> GSHMGSPNSPLKDSLRPKLSEEQQHIIAILLDAHHKTYDPTYADFRDFRPPVRMDGSTGSVTLDLSPLSMLPHLADLVSYSIQKVIGFAKMIPGFRDLTSDDQIVLLKSSAIEVIMLLSNQSFTMDDMSWDCGSQDYKYDVTDVSKAGHTLELIEPLIKFQVGLKKLNLHEEEHVLLMAICIVSPDRPGVQDAKLVEAIQDRLSNTLQTYIRCRHPPPGSHQLYAKMIQKLADLRSLNEEHSKQYRSLSFQPENSMKLTPLVLEVFGNEIS;> K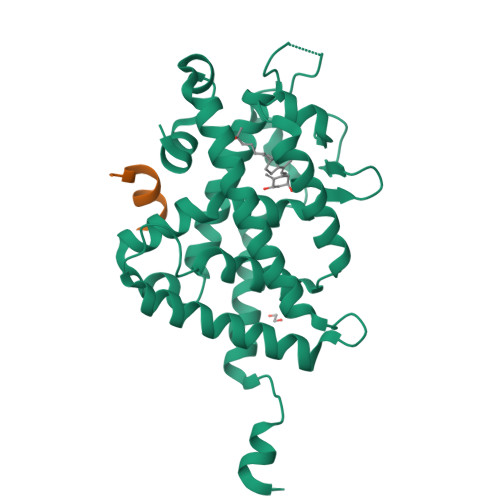NHPMLMNLLKDN>MGPGTWENMAFAQDSSAINNIDGYLSYTDWYRPYGTSQDGKTWYKTTAMDWRPLLMYIWPSKDVQAQFIKYFVNNGYENANYGLTKDTVANINKDTNTTVLANMAQNLRYVIEQSIAANKGTSKLANDINSFAATVPELSASSELSLQSMPNYRPDKSGTIDSDQVIFVNNNSKDPRKGNTSYADSNYRLMNRTINNQAGNNNSDNSPELLVGNDIDNSNPVVQAENLNWEYFLLNYGKLMGYNPDGNFDGFRVNAADNIDADVLDQMGQLMNDMYHTKGNPQNANDHLSYNEGYHSGAAQMLNEKGNPQLYMDSGEFYTLENVLGRANNRDN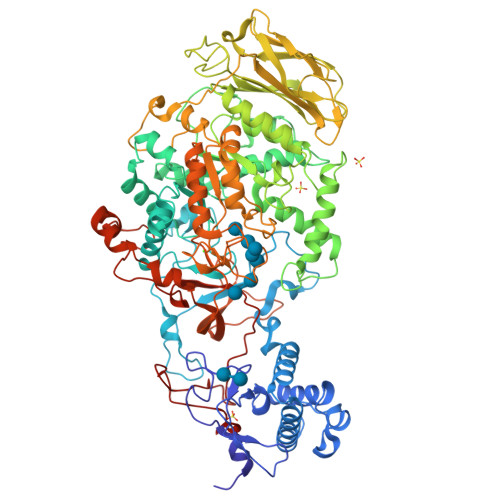IGNLITNSIVNRQNDTTENEATPNWSFVTNHDQRKNLINRLIIKDHSNIPDIMGSAYKVEYANQAWQEFYADQEKTNKQYAQYNVPAQYAILLSNKDTVPQVYYGDLYNETAQYMQEKSIYYDAITTLMRARKQFVSGGQTMTKLNNNLLASVRYGKGVVDANSNGTDKLSRTSGMAVLVGNDSNMAQQSVAINMGRAHANQQYRNLIDTTENGLTYDADNSENPAILTTDSNGILKVTVKGYSNPYVSGYLGVWVPVISGDQDVTTNASDVVANKEKTFESNAALDSHMIYEDFSLFQPEPTSVENHAYNVIAKNASLFSDLGITDFWMAPAYTPFGRSRYNEGYSMTDRYNLGTTANPTKYGSGEELANTIAALHKAGLKVQEDIVMNQMIGFSGQEAVTVTRTNNRGMQIHVNGQTYANQIYFAYTTGGGNGQETYGGKYLAELQKNYPDLFTTKAISTGVAPDPTVRINKWSAKYQNGTSLQNIGIGLAVKLANGDYAYLNSGDNKAFNTLLPTAIS[2x]>[4x]GAMDPEFMNKYQAVIIGFGKAGKTLAVTLAKAGWRVALIEQSNAMYGGTSINIGCIPTKTLVHDAQQHTDFVRAIQRKNEVVNFLRNKNFHNLADMPNIDVIDGQAEFINNHSLRVHRPEGNLEIHGEKIFINTGAQTVVPPIPGITTTPGVYDSTGLLNLKELPGHLGILGGGYIGVEFASMFANFGSKVTI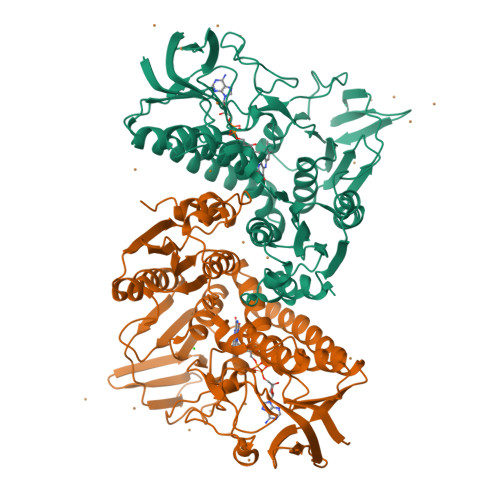LEAASLFLPREDRDIADNIATILRDQGVDIILNAHVERISHHENQVQVHSEHAQLAVDALLIASGRQPATASLHPENAGIAVNERGATVVDKRLHTTADNIWAMGDVTGGLQFTYISLDDYRIVRDELLGEGKRSTDDRKNVPYSVFMTPPLSRVGMTEEQARESGADIQVVTLPVAAIPRARVMNDTRGVLKAIVDNKTQRMLGASLLCVDSHEMINIVKMVMDAGLPYSILRDQIFTHPSMSESLNDLFSLVK> MSEIRKDTLKAILLELECHFTWNLLKEDIDLFEVEDTIGQQLEFLTTKSRLALYNLLAYVKHLKGQNKDALECLEQAEEIIQQEHSDKEEVRSLVTWGNYAWVYYHMDQLEEAQKYTGKIGNVCKKL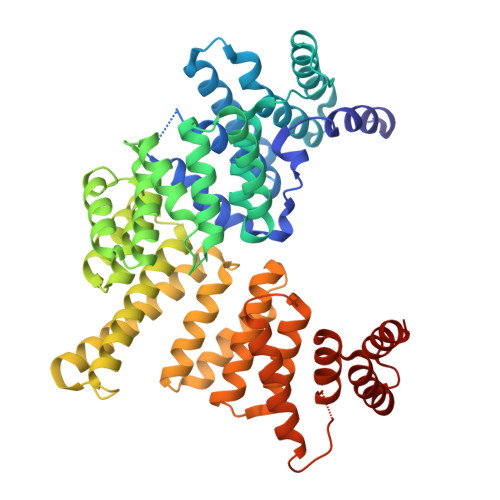SSPSNYKLECPETDCEKGWALLKFGGKYYQKAKAAFEKALEVEPDNPEFNIGYAITVYRLDDSDREGSVKSFSLGPLRKAVTLNPDNSYIKVFLALKLQDVHAEAEGEKYIEEILDQISSQPYVLRYAAKFYRRKNSWNKALELLKKALEVTPTSSFLHHQMGLCYRAQMIQIKKATHNRPKGKDKLKVDELISSAIFHFKAAMERDSMFAFAYTDLANMYAEGGQYSNAEDIFRKALRLENITDDHKHQIHYHYGRFQEFHRKSENTAIHHYLEALKVKDRSPLRTKLTSALKKLSTKRLCHNALDVQSLSALGFVYKLEGEKRQAAEYYEKAQKIDPENAEFLTALCELRLSI> MQPFGVLDRYIGKTIFTTIMMTLFMLVSLSGIIKFVDQLKKAGQGSYDALGAGMYTLLSVPKDVQIFFPMAA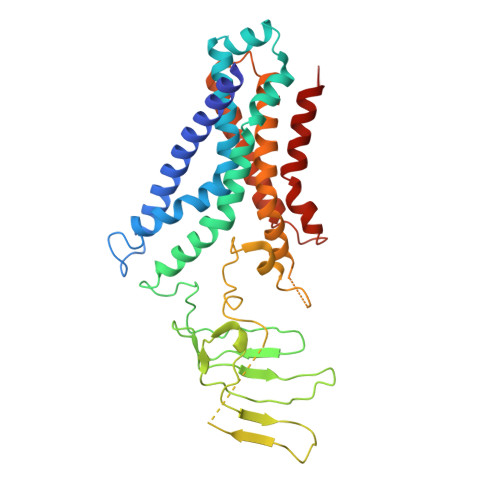LLGALLGLGMLAQRSELVVMQASGFTRMQVALSVMKTAIPLVLLTMAIGEWVAPQGEQMARNYRAQAMYGGSLLSTQQGLWAKDGNNFVYIERVKGDEELGGISIYAFNENRRLQSVRYAATAKFDPEHKVWRLSQVDESDLTNPKQITGSQTVSGTWKTNLTPDKLGVVALDPDALSISGLHNYVKYLKSSGQDAGRYQLNMWSKIFQPLSVAVMMLMALSFIFGPLRSVPMGVRVVTGISFGFVFYVLDQIFGPLTLVYGIPPIIGALLPSASFFLISLWLLMRKS>[4x]RPFLPKKKQQKDSLINLKIQKENPKVVNEINIEDLSLTKAAYCRCWRSKTFPACDGSHNKHNELTGDNVGPLILKKKEV

In humans, NEET proteins are represented by MiNT, localized inside the mitochondria, mitoNEET, and NAF-1, both anchored to the mitochondria outer membrane; with NAF-1 being also present on the surface of the endoplasmic reticulum and its mitochondria-associated membrane. NEET proteins harbor two [2Fe-2S] clusters with a unique 3Cys:1His coordination structure. Indeed, a growing amount of evidence demonstrate that NEET proteins play a significant role in Fe/Fe-S exchange between mitochondria and cytosol in cells. Here we report, for the first time, on a chemical compound, M1, that accelerates the dissociation of the [2Fe–2S] clusters of mNT and NAF-1 in a dose dependent manner.

In the M1-NAF-1 structure, determined at 1.74 Å resolution, only one extra density of M1 molecule is present in between two NAF-1 homodimers. The M1 molecule binds NAF-1 in the same area as observed in the mNT co-structure with carbonyl oxygens of the thiophene core forming salt bridges with Lys81 (equivalent of Lys55 of mNT) and does not interact with NAF-1 His114 (equivalent of His87 of mNT). However, the structure of M1-NAF-1 indicates that M1 is unable to form a hydrogen bond with Lys95 (equivalent of Lys68 of mNT). Although mNT and NAF-1 share a high percentage of sequence and structure homology, NAF-1 possesses a glutamate residue at position 85 (not alanine as for mNT). Consequently, Lys95 is able to form a salt bridge with Glu85 (2.7 Å distance). Moreover, the surface of mNT and NAF-1 show hydrophobic residues facing the hydrophobic moieties of M1 (<4.5 Å) suggesting hydrophobic interactions between M1 and the mNT/NAF-1 protein. A second important difference from the binding mode of furosemide to mNT is that the oxygen of the benzamide moiety of M1 molecule makes a hydrogen bond with mNT-Lys68 or shifts the position of NAF-1-Lys95. In the native protein, hydrogen bond formation between Lys55/Lys81 and His87/His114 (mNT/NAF-1), is critical for cluster stability with His87/His114 in effect performing a gatekeeper function which is compromised upon M1 binding to Lys55/Lys81 to result in higher lability of the bound clusters. Taken together the structures of M1-mNT/NAF-1 strongly suggest that in addition to His87/His114, interactions with Lys55/81 and cross-talk between the β-cap and the cluster binding area are also playing an important role in mNT and NAF-1 cluster lability/stability.> MHHHHHHHHGSMPTAAAPIISSVQKLVLYETRARYFLVGSNNAETKYRVLKIDRTEPKDLVIIDDRHVYTQQEVRELLGRLDLGNRTKMGQKGSSGLFRAVSAFGVVGFVRFLEGYYIVLITKRRKMADIGGHAIYKVEDTNMIYIPNDSVRVTHPDEARYLRIFQNVDLSSNFYFSYSYDLSHSLQYNLTVLRMPLEMLKSEMTQNRQESFDIFEDEGLITQGGSGVFGICSEPYMKYVWNGELLDIIKSTVHRDWLLYIIHGFCGQSKLLIYGRPVYVTLIARRSSKFAGTRFLKRGANCEGDVANEVETEQILCDASVMSFTAGSYSSYVQVRGSVPLYWSQDISTMMPKPPITLDQADPFAHVAALHFDQMFQRFGSPIIILNLVKEREKRKHERILSEELVAAVTYLNQFLPPEH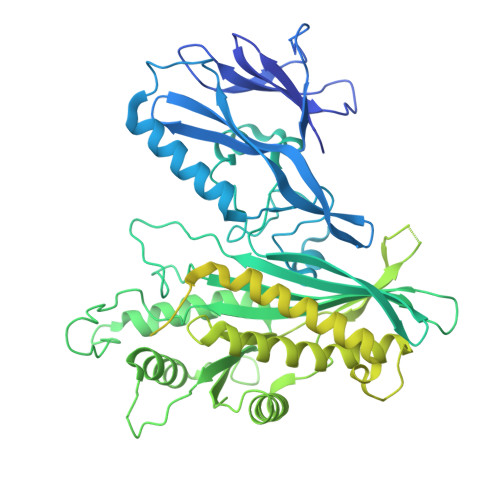TIVYIPWDMAKYTKSKLCNVLDRLNVIAESVVKKTGFFVNRPDSYCSILRPDEKWNELGGCVIPTGRLQTGILRTNCVDCLDRTNTAQFMVGKCALAYQLYSLGLIDKPNLQFDTDAVRLFEELYEDHGDTLSLQYGGSQLVHRVKTYRKIAPWTQHSKDIMQTLSRYYSNAFSDADRQDSINLFLGVFHPTEGKPHLWELPTDFYLHHKNTMRLLPTRRSYTYWWTPEVIKHLPLPYDEVICAVNLKKLIVKKFHKYEEEIDIHNEFFRPYELSSFDDTFCLAMTSSARDFMPKTVGIDPSPFTVRKPDETGKSVLGNKSNREEAVLQRKTAASAPPPPSEEAVSSSSEDDSGTDREEEGSVSQRSTPVKMTDAGDSAKVTENVVQPMKELYGINLSDGLSEEDFSIYSRFVQLGQSQHKQDKNSQQPCSRCSDGVIKLTPISAFSQDNIYEVQPPRVDRKSTEIFQAHIQASQGIMQPLGKEDSSMYREYIRNRYL>[8x]MTVQAQNIDAITAGAMPHEEPELTDGFHLVIDALKLNGIETIYNVPGIPITDLGRLAQAEGLRVISFRHEQNAGNAAAIAGFLTKKPGICLTVSAPGFLNGLTALANATTNCFPMILISGSSEREIVDLQQGDYEEMDQLAIAKPLCKAAFRVLHAADIGIGVARAIRAAVSGRPGGVYLDLPAKLFSQVIDADLGARSLVKVIDAAPAQLPAPAAIARALDVLKSAERPLIILGKGAAYAQADEAVRALVEESGIPYVPMSMAKGLLPDTHPLSAGAARSTALKDSDVVLLVGARLNWLLSHGKGKTWGEPGSKRFIQIDIEPREMDSNVEIVAPVVGDIGSCVEALLDGIRKDWKGAPSNWLETLRGKREANIAKMAPKLMKNSSPMCFHSALGALRTVIKERPDAILVNEGANTLDLARGIIDMYQPRKRLDVGTWGVMGIGMGFAVAAAVETGKPVLAVEGDSAFGFSGMEVETICRYELPVCIVIFNNNGIYRGTDTDPTGRDPGTTVFVKNSRYDKMMEAFGGVGVNVTTPDELKRAVDEAMNSGKPTLINAEIDPAAGSESGNIGSLNPQSTLKKK

Here, we employed structure-guided iterative saturation mutagenesis to convert oxalyl-CoA decarboxylase (OXC) from Methylobacterium extorquens into a glycolyl-CoA synthase (GCS) that allows for the direct condensation of the two C1 units formyl-CoA and formaldehyde. Previously, we showed that besides the decarboxylation of oxalyl-CoA into formyl-CoA, OXC from Methylorubrum extorquens (MeOXC) is also capable of catalyzing the acyloin condensation of formyl-CoA with various aldehydes, including formaldehyde. During catalysis, OXC and HACL both form the same α-carbanion/enamine intermediate. In HACL, this intermediate is generated through proton abstraction from formyl-CoA or by cleaving off the aldehyde moiety from a 2-hydroxyacyl-CoA thioester, whereas in OXC, this intermediate is formed by decarboxylation of oxalyl-CoA.

To gain insights into the specific active site topology of MeOXC, we solved the crystal structure of the enzyme at a resolution of 1.9 Å. Overall, the structure is very similar to that of OfOXC root-mean-square deviation (rmsd = 0.425 Å for 7230 aligned atoms). To increase the GCS activity of MeOXC, we sought to systematically alter the active site around the ThDP cofactor with ISM. Based on the crystal structure, we identified eight residues in the proximity of the ThDP cofactor as targets: I48, Y134, E135, A415, Y497, E567, S568, and I571. However, the catalytic efficiency of MeOXC with formaldehyde (kcat/KM = 2 M–1s–1) is far below that of RuHACL, which is the best performing HACL known to date (kcat/KM = 110 M–1s–1). Additionally, the KM for both substrates is extremely high (formaldehyde: 100 mM and formyl-CoA: 3 mM). In the first round of ISM (R1), libraries of positions 48 and 571 contained only variants with reduced activity, suggesting that the isoleucines in both of these positions are critical for catalysis.> GSEFGSGSNMSQWIRFRCSKIDEGGDWRPIVQFLRYQQIEFITFLGALKSFLKGTPKKNCLVFCGPANTGKSYFGMSFIHFIQGAVISFVNSTSHFWLEPL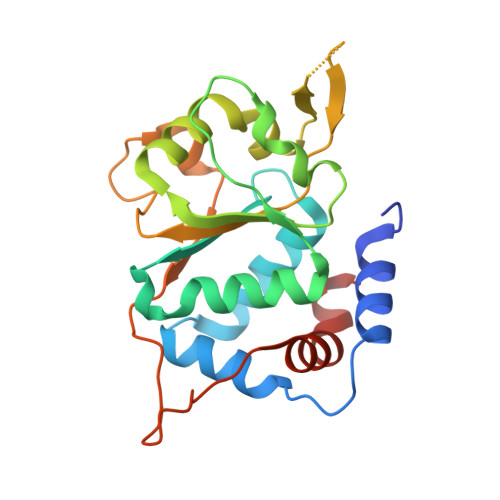TDTKVAMLDDATTTCWTYFDTYMRNALDGNPISIDRKHKPLIQLKCPPILLTTNIHPAKDNRWPYLESRITVFEFPNAFPFDKNGNPVYEINDKNWKCFFERTWSRLDLHE2-(acetyloxy)-3-methylbenzoic acid | C10 H10 O4 | 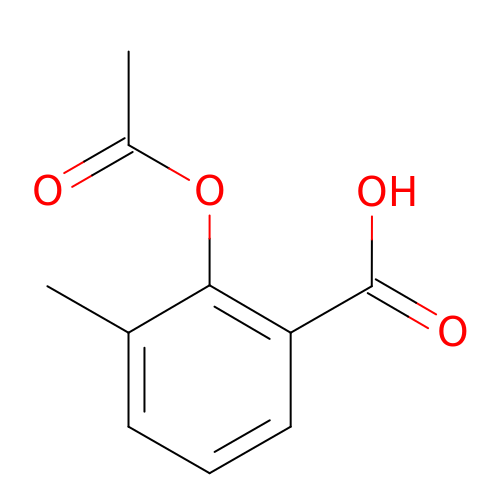XRBMKGUDDJPAMH-UHFFFAOYSA-N>[2x]SAMNNEGKALMAIKGSFSNLVNMLLDWDDVHNSDLCSWRGVFCDNVSYSVVSLNLSSLNLGGEISPAIGDLRNLQSIDLQGNKLAGQIPDEIGNCASLVYLDLSENLLYGDIPFSISKLKQLETLNLKNNQLTGPVPATLTQIPNLKRLDLAGNHLTGEISRLLYWNEVLQYLGLRGNMLTGTLSSDMCQLTGLWYFDVRGNNLTGTIPESIGNCTSFQILDISYNQITGEIPYNIGFLQVATLSLQGNRLTGR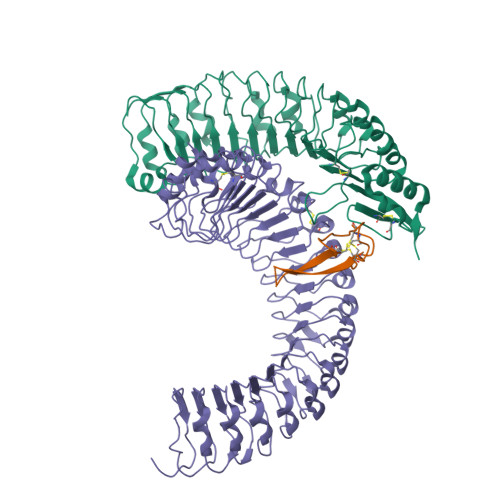IPEVIGLMQALAVLDLSDNELVGPIPPILGNLSFTGKLYLHGNMLTGPIPSELGNMSRLSYLQLNDNKLVGTIPPELGKLEQLFELNLANNRLVGPIPSNISSCAALNQFNVHGNLLSGSIPLAFRNLGSLTYLNLSSNNFKGKIPVELGHIINLDKLDLSGNNFSGSIPLTLGDLEHLLILNLSRNHLSGQLPAEFGNLRSIQMIDVSFNLLSGVIPTELGQLQNLNSLILNNNKLHGKIPDQLTNCFTLVNLNVSFNNLSGIVPPMKNFSRFAPASFVGNPYLCGNWVGSICGHHHHHH;>TSDSTAPSALIDGPQTGFTMTNDGARTEPDEQDAVYDIMRATGNDWAAAIPDVCRGRWHGIECMPDQDNVYHVVSLSFGALSDDTAFPTCDPQRSYVSESLTRLKHLKALFFYRCLGRAPQRIPAFLGRLGSSLQTLVLRENGFLGPIPDELGNLTNLKVLDLHKNHLNGSIPLSFNRFSGLRSLDLSGNRLTGSIPGFVLPALSVLDLNQNLLTGPVPPTLTSCGSLIKIDLSRNRVTGPIPESINRLNQLVLLDLSYNRLSGPFPSSLQGLNSLQALMLKGNTKFSTTIPENAFKGLKNLMILVLSNTNIQGSIPKSLTRLNSLRVLHLEGNNLTGEIPLEFRDVKHLSELRLNDNSLTGPVPFERDTVWRMRRKLRLYNNAGLCVNRDSDLDDAFGSKSGSTVRLCDAETSRPAPSGTVQHLSREEDGAL[2x];>[2x]TGSSLPDCSYACGACSPCKRVMISFECSVAESCSVIYRCTCRGRYYHVPSRA> GHMIKGEQKRYSEMTKEELQQEIAMLTEKARKAEQMGMVNEYAVYERKIAMAKAYMLN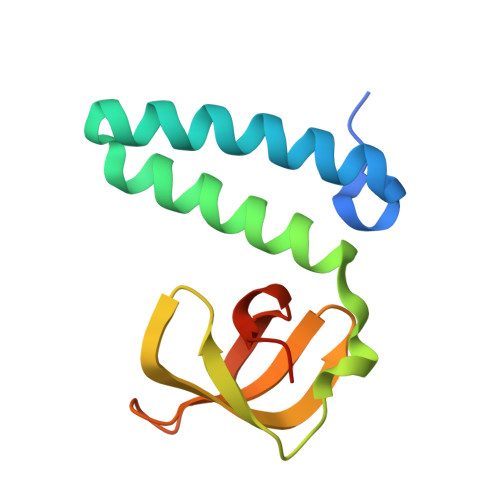PADFHPGEIYEIEGAPGEYFKVRYLKGVFAWGWRLKGNGEEEALPISLLRKPNLPQS> MTNKLFEHTVLYDSGDAFFELKGNASMKLSPKAAIEVCNEAAKKGLWILGIDGGHWLNPGFRIDSSASWTYDMPEEYKSKIPENN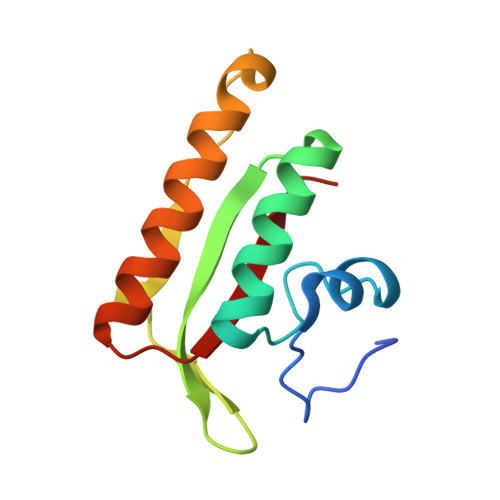RLAIENIKDDIENGYTAFIITLKM> PPGTPSRHEKSLGLLTTKFVSLLQEAKDGVLDLKLAADTLAVRQKRRIY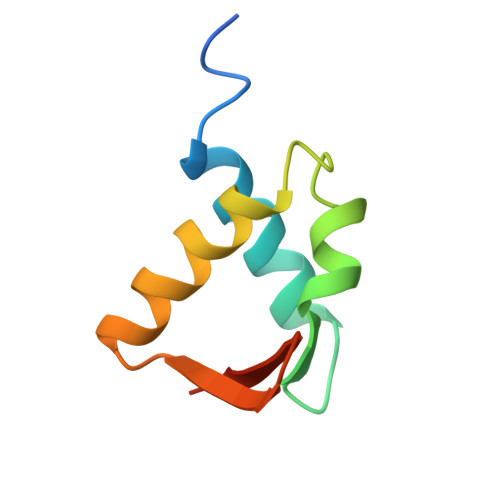DITNVLEGIGLIEKKSKNSIQWKGVGP> MGSSHHHHHHSSGGENLYFQGHMTETVTDQGKQRSSKLQKNEAAKDEQVEGKGKETLESGTDKSAEQNSSLLVGQPDVIDNDNVQTVDDFKNLMYKMQETRRAIVFALLNEKDLTKDDVEILKRAYEKLTDNQTHSFQREMCTLTTKLSVNIGDETRGLEKDLKYLDALMNIRREEPNLLWPIIMSRVDLFSILANYHPKGKETFLKEYEDTVKFLKTFISSEAITGKKPIFITDWDGTMKDYCSQYATNLQPVYSAVGMTRFAASFTRISAVLTAGPLRGPGILDLTAMPIDGPVMFSGSWGREWWLSGKRVVHQDGITDEG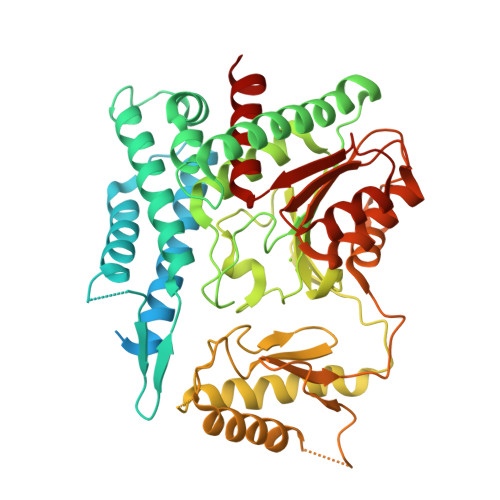FNALQRLDDEMKDLLHTSDYAPFALVGSGVQRKVDRLTLGVQTVCHHVTSELSNRYQMAVKERMHRVDPNSQILVFDPSTELEVEVVAHNSGIIWNKGNGVERLIKSLGDSLQSPGKILICGDTLSDIPMVRQAVKQNPDGVLAIFVGAKMSLREEVKQVIGDESRCCFVSCPDVIHAAMSQILNEHCIGK>MAHHHHHHMFISPQKIVPLSYNEFIRKVVSDHSIQEQEKEIRRLSQIVFGNQNQLANQLSQIHENPSFTKIISNTLTNSPESFAKLAGSKTFGIKNSKRKQAEKNISKLVEAIHKYADAVENSMGNIIKNH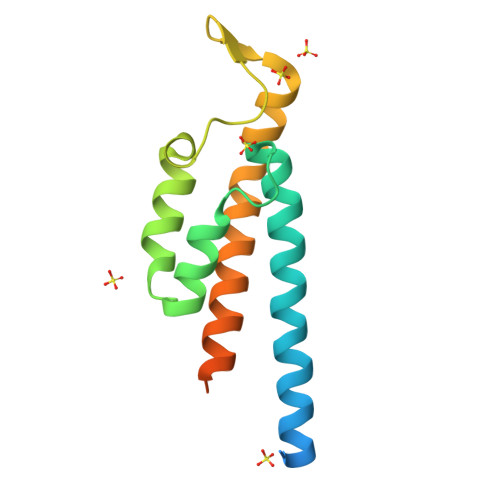NAEQKRLAQSVELPSD[2x]(2~{E},6~{E},10~{E})-3,7,11,15-tetramethylhexadeca-2,6,10,14-tetraen-1-ol 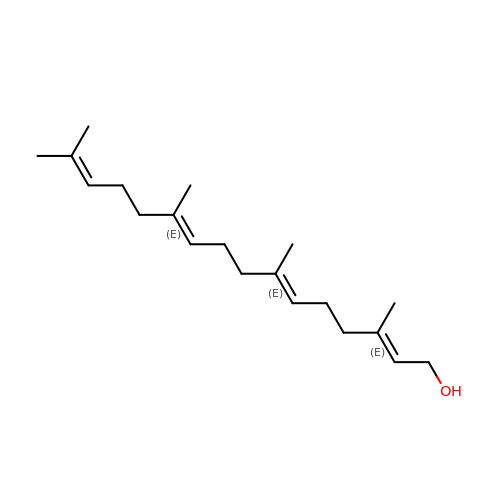| C20 H34 O | OJISWRZIEWCUBN-QIRCYJPOSA-N> MNKSQDEVKEDYFSIKKKKYNSLDCVLSPIVTRKKQESINSFQAGLQEDQNSTAVPESPFIRNCSETLNRSQHKILDHYFEYDYSLKKKIEKIKISLQNKTGTDSSQSLVQKRLDDLRKKTLIYKQFNIQKNNNNINNTGQFFIEKDKQNNLNLSQPHQIIKSKQGHKRSFTNTLYCSSNDKKIFNISSQKQNIKTVKQSNNSSMYEEQIKNDQNKKQNFNKQAKSERKQAEFCDLFYESMQKDAERQFKSNSDKSKSITQILENNCENAIVLLNHLIQILTDSIPISKNSILLDEKLSQCVNLSNNSKISQLMLVIQKLQGKISYYYNDFLKCIRMMKICKNFCQLFGTLKFKISCYKYIGLGFQRLNKPKVALVYFVKMLRQSWFLKQEDQEINSYDFIGMSYFYLGSIDKAYQYHQMM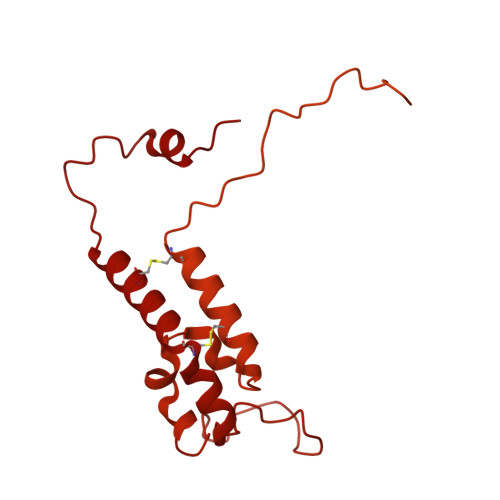IDGIKADEEVKKISNIMLKNRKYSNYPTLQNIRIIQETSDGQPLQKTIRKSKIINPQFQLTQQEWGENISSSEDEFELPQMQIAVKNAEEQTFQKKFLSTPWNDRFIQAQIHKLEIAQELNYNKFPIGLVFKNQSVLNFPNSSNQPQLVVGPYANKIYNQELSSTYSSRQRISHQTPNREFFNYHSQLQQVKEQTQLNQMKQQYNQIVDSIELANHLIVLKNLKKVKDLFQNLIPYLNEKYYNIKQQNTKSLKQQQNSFDAQNSNQSFLGLQNYSIQINGILNINNQTDEYVNNQSDRSYQQQSDKLKLLIKSKSRNHSKEINMTQNYFKSPSNESKQIKNLRVIVDNSNKKKAQQKLNQEFSMNFCESPKYDNSILSLFINKLSQESALRLEIRQIGSASRYQRKKQQKGKQRKEKYQKKQEENKLNIKQYKKERYNMALFFMANTAISVPSVLDTSPCMKQMLAYEDCVLDANVPQQEVIHPQWPTIWPRLLTDGKLLEFDKVPFHPENIYNYTYMRPLTKKNKQYLYECEEERFVFKACLRKVISLKKTDKHTSWDTAEVANLQLT> MAEEKLSARTQLPVSAESQKPVLKKAPEFPILEKQNWLIHLYYIQKDYEACKAVIKEQLQETHGLCEYAIYVQALIFRLEGNIQESLRLFQMCAFLSPQCADNLKQVARSLFLLGKHKAAIEVYNEAAKLNQKDWEICHNLGVCYIYLKQFDKAQDQLHNALHLNRHDLTYIMLGKIFLLKGDLDKAIEIYKKAVEFSPENTELLTTLGLLYLQLGIYQKAFEHLGNTLTYDPTNYKAILAAGSMMQTHGDFDVALTKYKVVACAVIESPPLWNNIGMCFFGKKKYVAAISCLKRANYLAPLDWKILYNLGLVHLTMQQYASAFHFLSAAINFQPKMGELYMLLAVALTNLEDSENAKRAYEEAVRLDKCNPLVNLNYAVLLYNQGEKRDALAQYQEMEKKVNLLKYSSSLEFDPEMVEVAQKLGA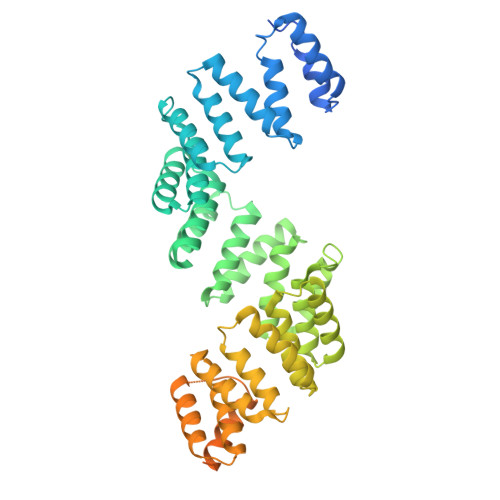ALQVGEALVWTKPVKDPKSKHQTASTSKAAGFQQPLGSNQALGQAMSSAATCRKLSSGAGGTSQLTKPPSLPLEPEPTVEAQPTEASAQTREK> MHHHHHHANIDESKIKDTVDDLIQPLMQKNNIPGMSVAVTVNGKNYIYNYGLAA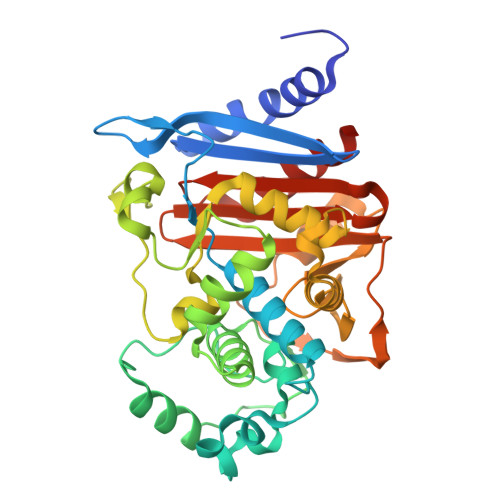KQPQQPVTENTLFEVGSLSKTFAATLASYAQVSGKLSLDQSVSHYVPELRGSSFDHVSVLNVGTHTSGLQLFMPEDIKNTTQLMAYLKAWKPADAAGTHRVFSNIGTGLLGMIAAKSLGVSYEDAIEKTLLPQLGMHHSYLKVPADQMENYAWGYNKKDEPVHVNMEILGNEAYGIKTTSSDLLRYVQANMGQLKLDANAKMQQALTATHTGYFKSGEITQDLMWEQLPYPVSLPNLLTGNDMAMTKSVATPIVPPLPPQENVWINKTGSTNGFGAYIAFVPAKKMGIVMLANKNYSIDQRVTVAYKILSSLEGNK In humans, ELAC2 carries out 3′ end processing of both nucleus-encoded (nu-tRNAs) and mitochondria-encoded (mt-tRNAs) tRNAs. ELAC2 is self-sufficient for processing of nu-tRNAs but requires TRMT10C and SDR5C1 to process most mt-tRNAs. The SDR5C1 tetramer forms a base to which TRMT10C is anchored through its ‘adapter helix’ and, together, they form a platform that binds the pre-tRNA substrate through interactions with all four tRNA subdomains. ELAC2 folds into two β-lactamase domains (N-terminal domain (NTD) and endonuclease domain), which form extensive interactions with the pre-tRNA through the acceptor stem, T-arm and 3′ trailer.

To determine the molecular basis of tRNA recognition and 3′ processing by ELAC2, we reconstituted RNase Z with either the canonical pre-mt-tRNAGln (mt-RNase ZGln) or the highly degenerated pre-mt-tRNATyr substrate (mt-RNase ZTyr) and a catalytically inactive variant of ELAC2 harboring an Asp550Asn substitution (ELAC2mut)59. The mt-RNase ZTyr complex was reconstituted by first incubating a 5′ leaderless pre-mt-tRNATyr substrate with TRMT10C–SDR5C1, followed by the addition of ELAC2mut. We then determined the structures of mt-RNase ZGln and mt-RNase ZTyr using single-particle cryo-EM at global resolutions of 3.4 and 3.2 Å, with the ELAC2 region at 4.0 and 3.6 Å after focused refinement, respectively. The structure of mt-RNase ZTyr reveals how TRMT10C and SDR5C1 facilitate processing of structurally degenerate mt-tRNAs. Overall, interactions between ELAC2 and pre-tRNATyr involve largely the same ribose phosphate interactions in the acceptor–T-arm minihelix and the 3′ trailer as observed in mt-RNase ZGln. However, the tRNA elbow structure that is recognized by ELAC2 in canonical tRNAs is absent in mt-tRNATyr, as no stable tertiary interactions are formed between the D-loop and T-loop. This results in a higher structural flexibility in the elbow region of pre-mt-tRNATyr compared to pre-mt-tRNAGln, with the D-loop and A56 and A57 at the tip of the T-loop poorly resolved in the EM density. The structure of mt-RNase ZTyr shows that TRMT10C–SDR5C1, in addition to its structural support for the overall tRNA fold, facilitates processing of such mt-tRNAs by stabilizing ELAC2 through direct protein–protein interactions with TRMT10C, which compensate for the loss of interactions between ELAC2 and the tRNA elbow. To better resolve the productive active-site conformation, we performed a three-dimensional (3D) variability analysis of mt-RNase ZTyr particles with respect to the ELAC2 conformational state. This resulted in a class where the pre-mt-tRNATyr adopts a ‘contracted’ conformation, allowing the RNA to be positioned in the ELAC2 active site.

>[4x]MAAACRSVKGLVAVITGGASGLGLATAERLVGQGASAVLLDLPNSGGEAQAKKLGNNCVFAPADVTSEKDVQTALALAKGKFGRVDVAVNCAGIAVASKTYNLKKGQTHTLEDFQRVLDVNLMGTFNVIRLVAGEMGQNEPDQGGQRGVIINTASVAAFEGQVGQAAYSASKGGIVGMTLPIARDLAPIGIRVMTIAPGLFGTPLLTSLPEKVCNFLASQVPFPSRLGDPAEYAHLVQAIIENPFLNGEVIRLDGAIRMQP;> SNAPRKDPLRHLRTREKRGPSGCSGGPNTVYLQVVAAGSRDSGAALYVFSEFNRYLFNCGEGVQRLMQEHKLKVARLDNIFLTRMHWSNVGGLSGMILTLKETGLPKCVLSGPPQLEKYLEAIKIFSGPLKGIELAVRPHSAPEYEDETMTVYQIPIHSEQRRGKHQPWQSPERPLSRLSPERSSDSESNENEPHLPHGVSQRRGVRDSSLVVAFICKLHLKRGNFLVLKAKEMGLPVGTAAIAPIIAAVKDGKSITHEGREILAEELCTPPDPGAAFVVVECPDESFIQPICENATFQRYQGKADAPVALVVHMAPASVLVDSRYQQWMERFGPDTQHLVLNENCASVHNLRSHKIQTQLNLIHPDIFPLLTSFRCKKEGPTLSVPMVQGECLLKYQLRPRREWQRDAIITCNPEEFIVEALQLPNFQQSVQEYRRSAQDGPAPAEKRSQYPEIIFLGTGSAIPMKIRNVSATLVNISPDTSLLLDCGEGTFGQLCRHYGDQVDRVLGTLAAVFVSHLHANHHTGLPSILLQRERALASLGKPLHPLLVVAPNQLKAWLQQYHNQCQEVLHHISMIPAKCLQEGAEISSPAVERLISSLLRTCDLEEFQTCLVRHCKHAFGCALVHTSGWKVVYSGDTMPCEALVRMGKDATLLIHEATLEDGLEEEAVEKTHSTTSQAISVGMRMNAEFIMLNHFSQRYAKVPLFSPNFSEKVGVAFDHMKVCFGDFPTMPKLIPPLKALFAGDIEEMEERREKRELRQVRAALLSRELAGGLEDGEPQQKRAHTEEPQAKKVRAQ;> SNAAATREFIEMWRLLGREVPEHITEEELKTLMECVSNTAKKKYLKYLYTKEKVKKARQIKKEMKAAAREEAKNIKLLETTEEDKQKNFLFLRLWDRNMDIAMGWKGAQAMQFGQPLVFDMAYENYMKRKELQNTVSQLLESEGWNRRNVDPFHIYFCNLKIDGALHRELVKRYQEKWDKLLLTSTEKSHVDLFPKDSIIYLTADSPNVMTTFRHDKVYVIGSFVDKSMQPGTSLAKAKRLNLATECLPLDKYLQWEIGNKNLTLDQMIRILLCLKNNGNWQEALQFVPKRKHTGFLEISQHSQEFINRLKKAKT> MPSTSPADKDVPMSILHTHGLSYVNWCMSLAPGLLVFEGFFRARYYRSRVPPSR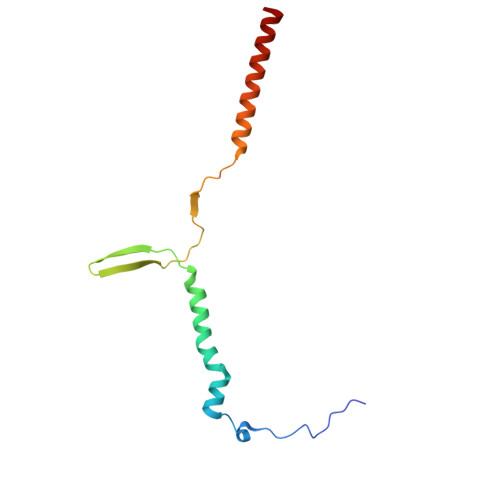TVLMNGLKMRMFSLARQQAPKIVHKPVLSPIPEHLRLVKNVAQVQIDMLKLLNAQAAK>MEEKVGNLKPNMESVNVTVRVLEASEARQIQTKNGVRTISEAIVGDETGRVKLTLWGKHAGSIKEGQVVKIENAWTTAFKGQVQLNAGSKT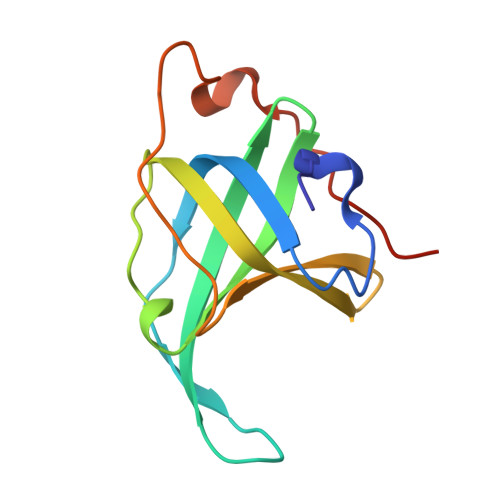KIAEASEDGFPESSQIPENTPTAPQQMR[2x]>AHMFMAENRLQLQKGSAEETIERFYNRQGIETIEGFQQMFVTKTLNTEDTDEVKILTIWESEDSFNNYLNSDVFKEAHKNVRLKSDDDGQQSPILSN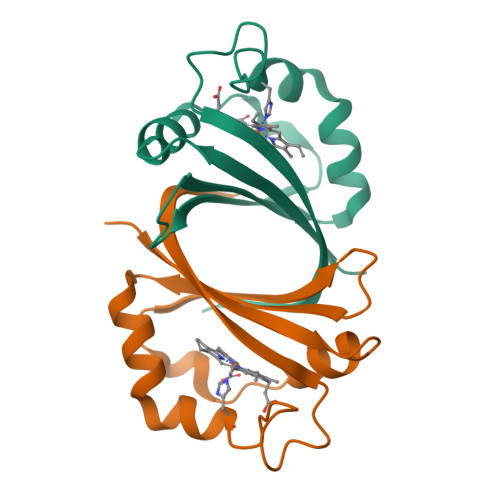KVFKYDIGYHYQK[2x]> KKISNPIIP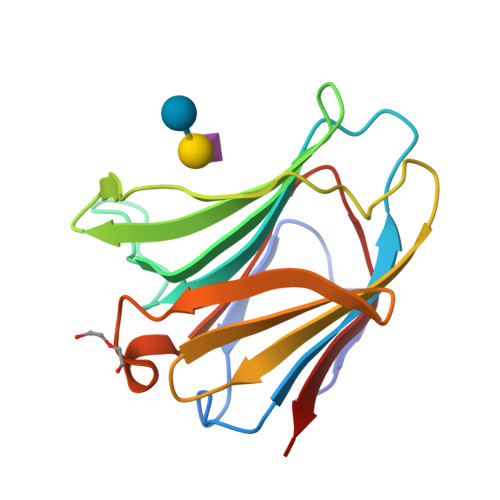YVGTILGGLVPGELIVLHGSIPDDADRFQVDLQCGSSIKPRADVAFHFNPRFKWSGCVVCNTLEREKWGWEEITYEMPFQKGRPFEIVIMILKDKFQVSVNKKHLLLYNHRISLERIDTLGIYGKVQIKSIEFVS Quantitative data about starch phosphorylase protein abundance and enzyme activity are lacking and no crystal structure of a plastidic plant starch phosphorylase has been reported so far. It is known that starch phosphorylases are members of the CAZy GT35 family of glycosyltransferases and catalyze the reversible transfer of glucosyl residues from a glucose donor onto the non-reducing end of an α-glucan chain. While Pho2 is localized in the cytosolic compartment, Pho1 is a true starch phosphorylase that acts on starch in the plastids of the plant cell. We determined the crystal structures of HvPho1, the first crystal structure of a plastidic plant starch phosphorylase. A native structure of HvPho1 and two complexes with acarbose and maltotetraose were solved and refined to resolutions of 2.7 Å, 2.9 Å and 3.0 Å respectively.

The third crystal, soaked with acarbose and G1P, has no ordered electron density for either substrate in the active site. Some disordered electron density is present there, and two fragments in each monomer have been interpreted as glucose molecules in our final model, but they probably represent the average electron density of a mixture of many species, possibly including solvent water and glycerol. Correspondingly, the 422–427 loop is in the open conformation as in the native structure. Acarbose molecules were modeled, one for each monomer, in arc-shaped electron density going through a gate formed by Tyr900 and Tyr905 and adjacent to the active site. This gate is already formed, albeit unoccupied, in the native structure. The acarbose molecules have their non-reducing ends overlapping with the position of the glucoses in subsite +4 in the maltotetraose soak. Together, these two crystal structures define a path for the acceptor maltooligosaccharide from subsite +1 to subsite +7, at which point the maltooligosaccharides would extend into the solvent.

>[2x]MRSVASDREVRGPASTEEELSAVLTSIDSSAIASNIQHHADFTPLFSPEHSSPLKAYHATAKSVFDSLIMNWNATYDYYNKVNAKQAYYLSMEFLQGRALTNAIGNLELTGQYAEALKQLGHNLEDVASQEPDPALGNGGLGRLASCFLDSLATLNYPAWGYGLRYRYGLFKQIITKDGQEEVAENWLEMGNPWEIVRNDVSYPVKFYGKVVEGTDGRKHWIGGENIKAVAHDVPIPGYKTKTTNNLRLWSTTVPSQNFDLGAFNAGDHAKANEAHLNAEKICHVLYPGDESSEGKILRLKQQYTLCSASLQDIISRFESRAGDSLNWEDFPSKVAVQMNDTHPTLCIPELMRILMDIKGLSWNEAWSITERTVAYTNHTVLPEALEKWSLDIMQKLLPRHVEIIETIDEELMNNIVSKYGTADISLLKQKLKDMRILDNVDLPASVAKLFIKPKEKRGKLLVESLESIAEADEKTESQEVENILSETTEKKAESDSEEAPDAEKEDPEYELDPFAKYDPQFPRVVRMANLCVVGGHSVNGVAEIHSEIVKQDVFNSFYEMWPTKFQNKTNGVTPRRWIRFCNPELSTIISKWIGSDDWILNTDKLAGLKKFADDEDLQSEWRTAKRNNKMKVVSLIRDKTGYIVSPDAMFDVQVKRIHEYKRQLLNILGIVYRYKKMKEMSAKDRRKSFVPRVCIFGGKAFATYVQAKRIVKFITDVAATVNYDPDIGDLLKVVFVPDYNVSVAETLIPASELSQHISTAGMEASGTSNMKFAMNGCLLIGTLDGANVEIREEVGEENFFLFGAHAPEIAGLRQERAEGKFVPDLRFEEVKEYVRSGVFGTSNYDELMGSLEGNEGYGRADYFLVGKDFPSYIECQEKVDEAYRDQKLWTRMSILNTAGSPKFSSDRTIHEYAKDIWDISPVIMPTFPDIENLYFQG Halohydrin dehalogenases (HHDHs; also, haloalcohol dehalogenases or epoxidases, halohydrin hydrogen-halide-lyases) are biotechnologically relevant enzymes for the production of chiral epoxides and β-substituted alcohols. In their natural function, they catalyze the reversible dehalogenation of vicinal haloalcohols with formation of the corresponding epoxides. HHDHs possess a catalytic triad composed of serine, tyrosine and arginine. Protein engineering of halohydrin dehalogenase HheG for thermostabilization revealed several residues with positive impact on the apparent melting temperature.

Superimposition revealed that mutations T123G and T123W have no effect on the overall fold of the protein or on the position and orientation of the catalytic residues S152, Y165 and R169. A more thorough analysis of the variants shows that mutation of T123 to glycine or tryptophan leaves backbone hydrogen bonds to G102 and K119 unaltered, whereas side chain-specific contacts to L103, K119 and N124 are abolished. In the T123W variant, new hydrophobic interactions of the tryptophan side chain with T75, L103 and M127 are established, which may contribute to the increased thermostability of this variant. The loop of variant T123W displays a significantly higher mobility compared to wild-type HheG and variant T123G, for which a lower loop mobility has been obtained. In summary, the observed average loop position of variant T123W is very similar to the one found in HheG wild-type, while the loop mobility is significantly increased in this variant. Hence, also the ability of the T123W loop to (partially) close the active site cleft is increased compared to wild-type HheG. While the loop consisting of residues 39 to 47 leads to denser packing and increased buried surface area in T123G, it is more flexible in T123W. For the latter variant, the crystal structure indicates specific new interactions of the tryptophan with nearby residues, which might contribute to a higher thermostability of T123W. Moreover, the flexible loop could provide M45 as additional interaction partner for W123. In contrast, exchange of T123 by an aromatic residue yielded the highest gain in thermostability with 12–14 °C increase in Tm.

>[10x]ENRPVALITMATGYVGPALARTMADRGFDLVLHGTAGDGTMVGVEESFDSQIADLAKRGADVLTISDVDLTTRTGNQSMIERVLERFGRLDSACLVTGLIVTGKFLDMTDDQWAKVKAWNLDMVFHGLQAVLPPMVAAGAGQCVVFTSATGGRPDPMVSIYGGTRAGANGIVRAVGLEHARHGVQVNAIGTNYMDFPGFLKASRADGDPERRAMIEAQVPLRRLGTMDELSSVTAGLLDGSNRFQTGQFFDFSGGWGA> AGYKTCPKVKPDMLNVHLVPHTHDDVGWLKTVDQYFYGIYNNIQPAGVQYILDSVISSLLANPTRRFIYVEIAFFSRWWRQQTNATQKIVRELVRQGRLEFANGGWVMNDEATTHYGAIIDQMTLGLRFLEETFGSDGRPRVAWHIDPFGHSREQASLFAQMGFDGFFFGRLDYQDKKVRKKTLQMEQVWRASTSLKPPTADLFTSVLPNMYNPPEGLCWDMLCADKPVVEDTRSPEYNAKELVRYFLKLATDQGKLYRTK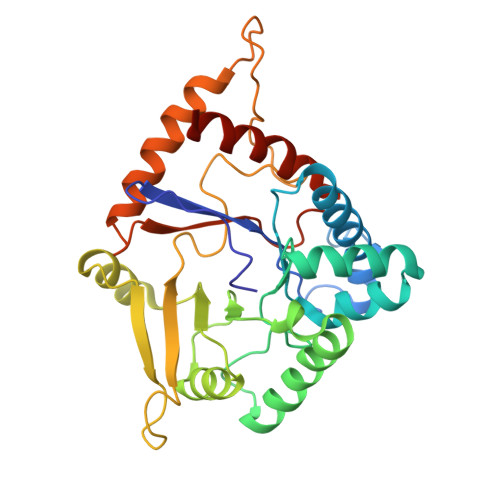HTVMTMGSDFQYENANTWFKNLDKLIQLVNAQQRANG>[4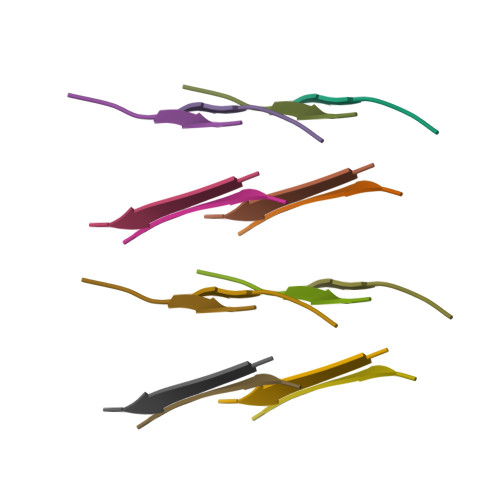x]GGYVLG>[2x]G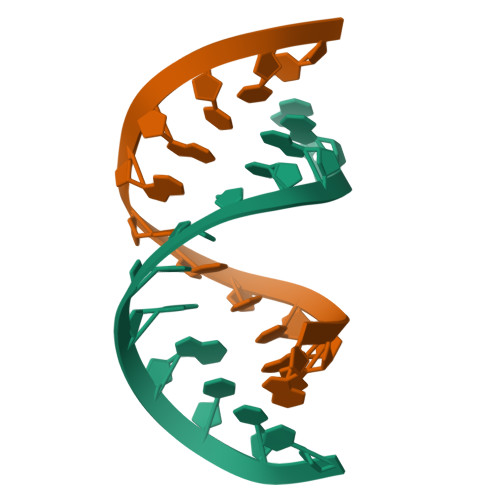GACUUUGGUCC>MHHHHHHENLYFQGSH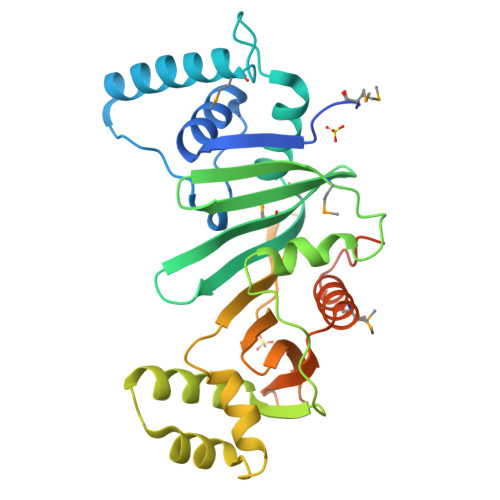MGPNAVELTTDQAWCLADVLGAGSYPWVLAITPPYSDHSQRSAFLAAQSAELTRMGVVNSAGAVDPRVAQWITTVCRATQWLDLRFVSGPGDLLRGMVARRSEETVVALRNAQLVTFTAMDIGHQHALVPVLTAGLSGRKPARFDDFALPAAAGARADEQIRNGAPLAEVLEFLGVPPSARPLVESVFDGRRTYVEIVAGEHRDGHRVTTEVGVSIIDTPHGRILVHPTKAFDGEWISTFTPGSADAIAMAVERLTASLPSGSWFPDQPLTRDFDEDAATHREPVLQRRTQKA[2x]>MELWLVRHGETLWNREGRLLGWTDLPLTAEGEAQARRLKGALPSLPAFSSDLLRARRTAELAGFSPRLYPELREIHFGAMEGALWETLDPRYKEALLRFQGFHPPGGESLSAFQE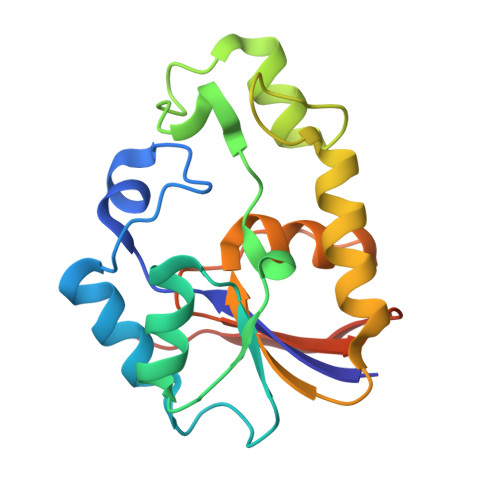RVFRFLEGLKAPAVLFTHGGVVRAVLRALGEDGLVPPGSAVAVDWPRRVLVRLALDGEEATG[2x]>[2x]MSRLDKSKVINSALELLNEVGIEGLTTRKLAQKLGVEQPTLYWHVKNKRALLDALAIEMLDRHHTHFSPLEGESWQDFLRNNAKSFRNALLSHRDGAKVHLGTRPTEKQYETLENQLAFLTQQGFSLENALYALSAVGHFTLGSVLEDQEHQVAKEERETPTTDSMPPLLRQAIELFDHQGAEPAFLHGLESLIRGFEVQLTALLQIV

Eponymous TetR is a homodimeric α-helical protein, and each monomer comprises 10 α-helices. The tertiary structure of TetR family members consists of two domains: an N-terminal nucleotide-binding domain (NBD) and a C-terminal effector-binding domain (EBD) that also contains the dimerization interface. In the absence of its natural ligand tc, TetR binds to the DNA tetO operator sequence and thereby represses downstream genes. Upon tc binding to the EBD, TetR undergoes an allosteric rearrangement that increases the separation of the NBDs, abolishes tetO operator binding and alleviates gene repression.

The crystal structure of TetR in complex with the 43-nucleotide-long TetR-binding RNA aptamer K1 was determined at 2.7 Å resolution. The complex consists of one TetR dimer bound to a single aptamer. In the complex, TetR adopts a conformation that is highly similar to the conformation that TetR adopts for DNA binding and which has been extensively characterized before. The aptamer adapts a hairpin-like L-shaped structure in the complex. The two arms of the L-shape consist of a 3 bp-long closing stem P1 and a 4 bp-long P2 stem. Although in the complexed aptamer, the P2 stem is closed-off by an apical GAAA loop on one side, no density is visible for the central two nucleotides of the tetraloop. Overall, 36 nucleotides, i.e. nucleotides 4–22 and 25 to 41, of the 43-nucleotide-long aptamer K1 could be modeled with confidence. A direct consequence of the symmetry disparity between dimeric TetR and the monomeric aptamer is that the two NBDs of TetR interact with two different aptamer surface patches. Six TetR residues, i.e. Arg28, Arg28′, Gln38, Tyr42, Tyr42′ and Lys46, are involved in sequence-specific interactions with the aptamer. Arg28 and Arg28′ each form a bidental hydrogen-bonding interaction with a guanine nucleobase, specifically G31 in case of Arg28 and G12 in case of Arg28′.> SNAEREEEP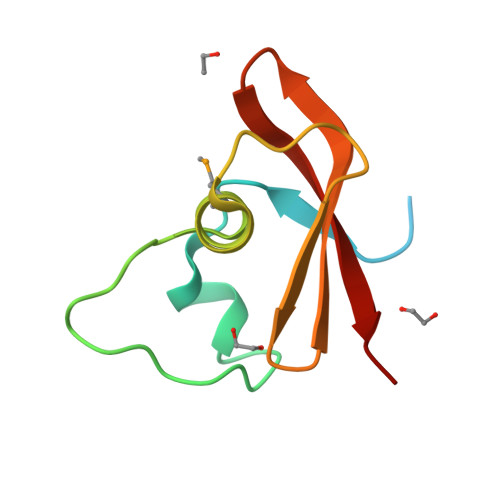AVQGNPDESLTVEGALEYVELAPQLNLPQQEEDADFHTVAGLIMEELQTIPDVGDFADFHGWRFEVVEKEGQRIERVKITKLP> MEFGFWSALYIFVLTCFLGYELITRVPVILHTPLMSGSNFIHGVVVVGAMVVLGHAE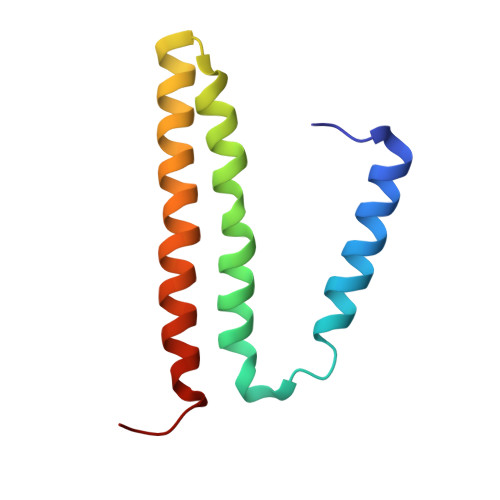TGLEKLIGFLGVILGAANAAGGYAVTVRMLEMFERKP2-[4-(4-CYANOPHENYL)-3-{[4-(PYRIDIN-2-YL)PIPERAZIN-1-YL]METHYL}PHENOXY]-N-METHYLACETAMIDE 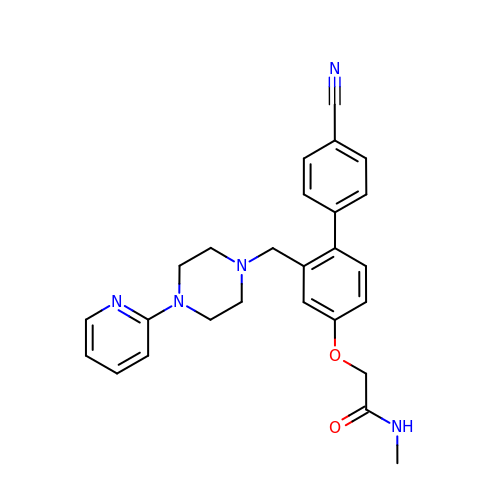| C26 H27 N5 O2 | MATAFJDAEJJYTE-UHFFFAOYSA-N> CVIFPVEIDVSQTIIRDCQVDKQTRELVYINKIMNTQLTKPVLMMFNISGPIRSVTRKNNNLRDRIKSKPDEQFDQLEKDYSDQMDGFHDSIKYFKDEHYSVSCQNGSVLKSKFAKILKSHDYTDKKSIEAYE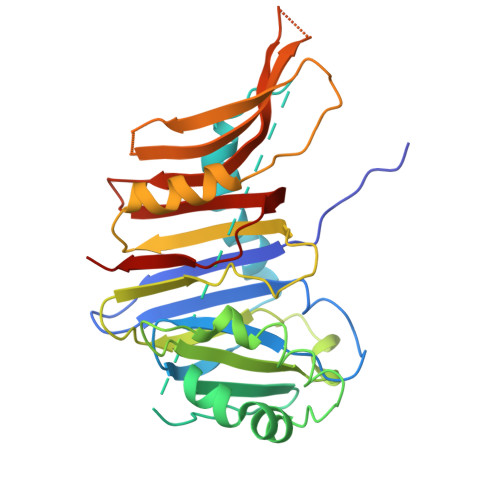KYCLPKLVDERNDYYVAVCVLKPGFENGSNQVLSFEYNPIGNKVIVPFAHEINDTGLYEYDVVAYVDSVQFDGEQFEEFVQSLILPSSFKNSEKVLYYNEASKNKSMIYKALEFTTESSWGKSEKYNWKIFCNGFIYDKKSKVLYVKLHNVTSALNKNVILNTIK6-methoxyquinoline-3-carboxylic acid | C11 H9 N O3 | 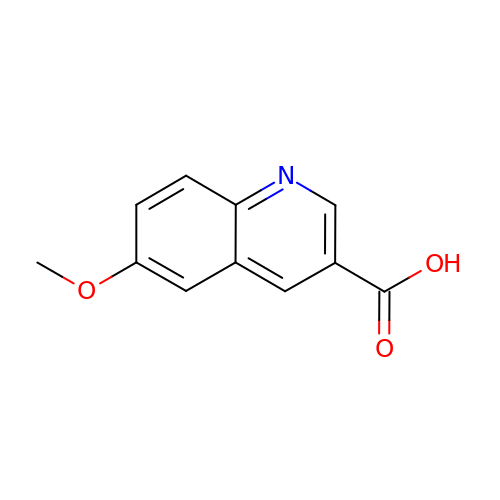QSFFBQNKTUMKNW-UHFFFAOYSA-N> MAGLPNSSNALQQWHHLFEAEGTKRSPQAQQHLQQLLRTGLPTRKHENWKYTPLEGLINSQFVSIAGEISPQQRDALALTLDSVRLVFVDGRYVPALSDATEGSGYEVSINDDRQGLPDAIQAEVFLHLTESLAQSVTHIAVKRGQRPAKPLLLMHITQGVAGEEVNTAHYRHHLDLAEGAEATVIEHFVSLNDARHFTGARFTINVAANAHLQHIKLAFENPLSHHFAHNDLLLAEDATAFSHSFLLGGAVLRHNTSTQLNGENSTLRINSLAMPVKNEVCDTRTWLEHNKGFCNSRQLHKTIVSDKGRAVFNGLINVAQHAIKTDGQMTNNNLLMGKLAEVDTKPQLEIYADDVKCSHGATVGRIDDEQIFYLRSRGINQQDAQQ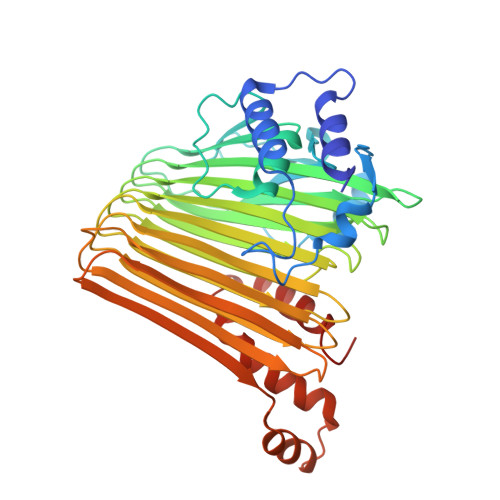MIIYAFAAELTEALRDEGLKQQVLARIGQRLPGGAR>MERTFLMIKPDAVQRNLIGEVISRIERKGLKLVGGKLMQVPMELAETHYGEHQGKPFYNDLISFITSAPVFAMVVEGEDAVNVSRHIIGSTNPSEASPGSIRGDLGLTVGRNIIHGSDSLESAEREINLWFNENEITS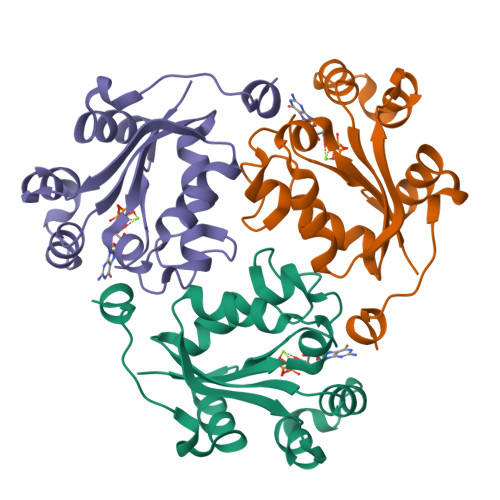YASPRDAWLYELEHHHHHH[2x]>MALNTIEDAVKLLQECKKIIVLTGAGVSVSCGIPDFRSRDGIYARLAVDFPDLPDPQAMFDIEYFRKDPRPFFKFAKEIYPGQFQPSLCHKFIALSDKEGKLLRNYTQNIDTLEQVAGIQRIIQCHGSFATASCLICKYKVDCEAVRGDIFNQVVPRCPRCPADEPLAIMKPEIVFFGENLPEQFHRAMKYDKDEVDLLIVIGSSLKVRPVALIPSSIPHEVPQILINREPLPHLHFDVELLGDCDVIINELCHRLGGEYAKLCCNPVKLS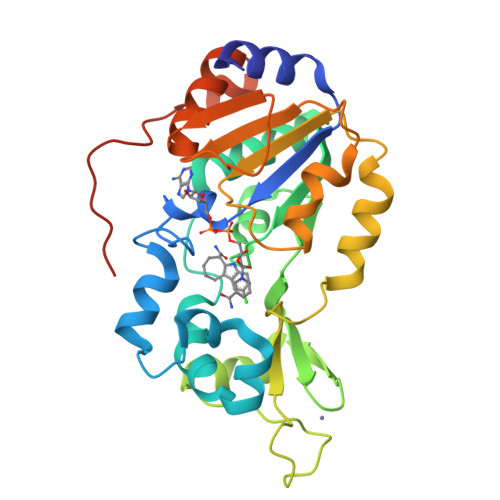EITEKPPREGHHHHHH[2x]> GGAGHVPEYF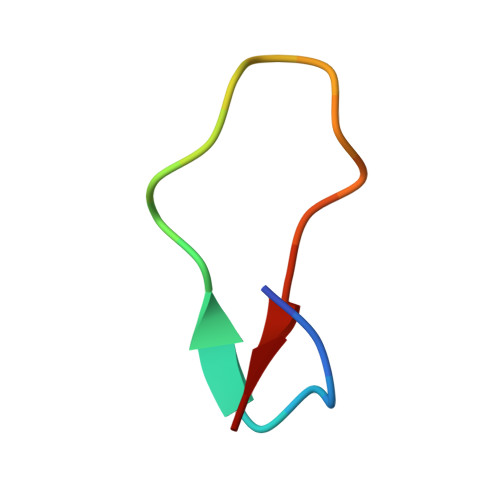VGIGTPISFYG> MRATLRQCNVFDPAFMRKVKRTLSAYKGSMETSAKKSMSREAFVDIDEKGAAWYLGHMQSAANMLADKVKDADFILEIRDARLPFTTENPNIRKLTAGKPRLIIFNKAELSNEDSNRAIQEYYERNGAFALFTSARRCWRDVVEAVQRFTTHILPPLPYKTVAHVGLVVGMPNVGKSTLINSLRLAHEYQFHREDFRRSRSPETVSITPGTTRGMKLVPLSKDPPVVLYDTPGLTLPGCFTKESGLKLAACGIIPTNDVSLPQGMVARYIYDILVASGSSEHMAECLHLPRVPISFDDCVAMICERSGTSGQTEMGNLDPVRAHRFFVHDFIMGNLGKITLDVLPRRLLRSSQSSIPLLESGSSTAATDGAQAAAGDDDGYAWTHHVETSDVVERYPDHMRDVLQSLKGPLHHDG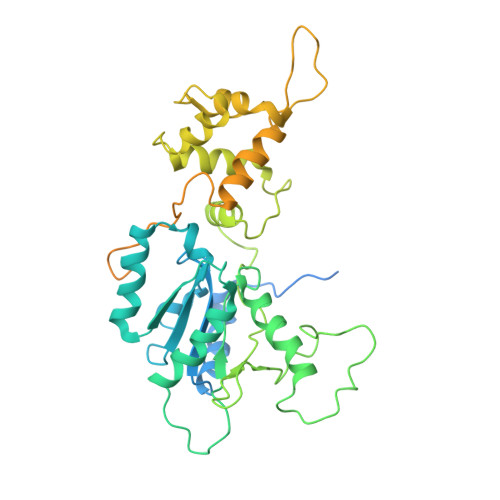VPRRHQAPSVKNLDSPSDCTVISRKKGPISRVTAFDEQLKRHTRLTPGR>RPRVYVDVREERSPVPSILESLGVQVIPKQLPMGDYLVSDSIIVERKTSSDFAKSLFDGRLFEQASRLAEHYETVFIIVEGPPVPRRYRGRERSLYAAMAALQLDYGIRLMNTMDPKGTALVIESLARLSTREGGQRIVIHKKPRLSDVREWQLYILQSF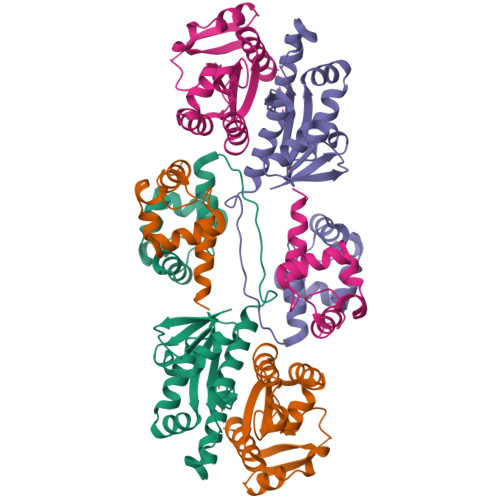PGIGRRTAERILERFGSLERFFTASKAEISKVEGIGEKRAEEIKKILMTPYKRS[4x]>[2x]QDNSRYTHFLTLHYDAKPQGRDDRYCESIMRRRGLTSPCKDINTFIHGNKRSIKAICENKNGNPHRENLRISKSSFQVTTCKLHGGSPWPPCQYRATAGFRNVVVACENGLPVHLDQSIFR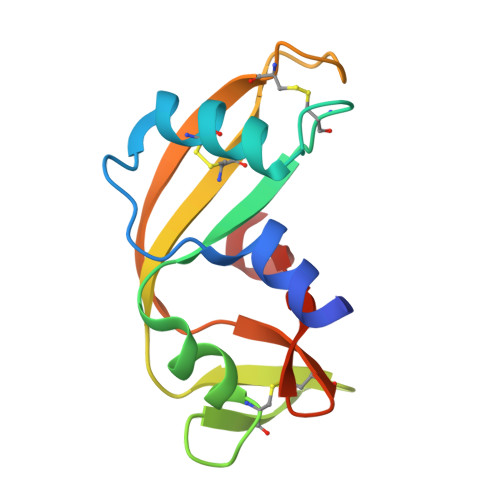RP(6~{R})-6-[[3,4-bis(oxidanylidene)-2-[[4-(trifluoromethyloxy)phenyl]amino]cyclobuten-1-yl]amino]-~{N}-oxidanyl-heptanamide 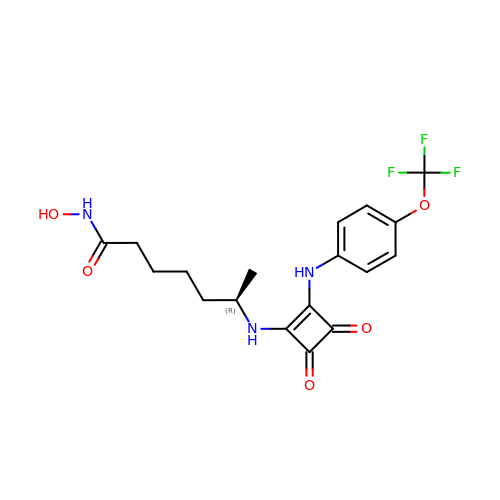| C18 H20 F3 N3 O5 | WFKNHSZTAURQLQ-SNVBAGLBSA-N> VLLESEQFLTELTRLFQKCRTSGSVYITLKKYDGRTKPIPKKGTVEGFEPADNKCLLRATDGKKKISTVVSSKEVN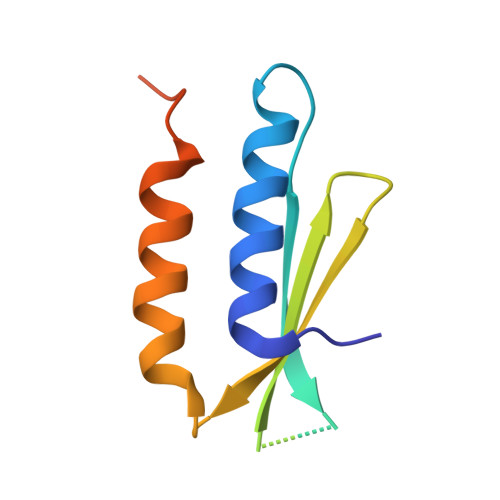KFQMAYSNLLRANMDGLKKRDKKNKTKKTK>GPHMPGSR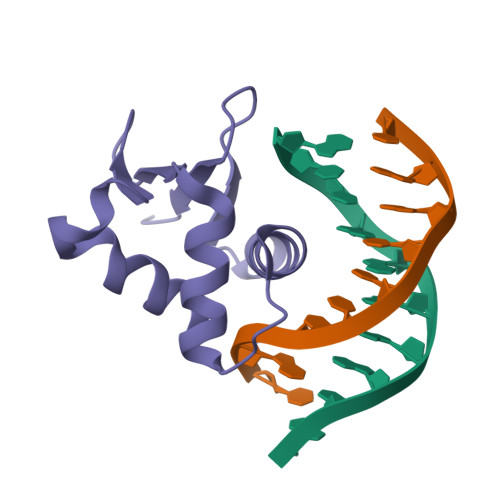QIQLWHFILELLRKEEYQGVIAWQGDYGEFVIKDPDEVARLWGVRKCKPQMNYDKLSRALRYYYNKRILHKTKGKRFTYKFNFNKLVLVNYPFIDVGLAGGAVPQSAPPVPSGGS[4x]1-{3-[7-(difluoromethyl)-6-(1-methyl-1H-pyrazol-4-yl)-3,4-dihydroquinolin-1(2H)-yl]-1-(oxan-4-yl)-1,4,6,7-tetrahydro-5H-pyrazolo[4,3-c]pyridin-5-yl}ethan-1-one 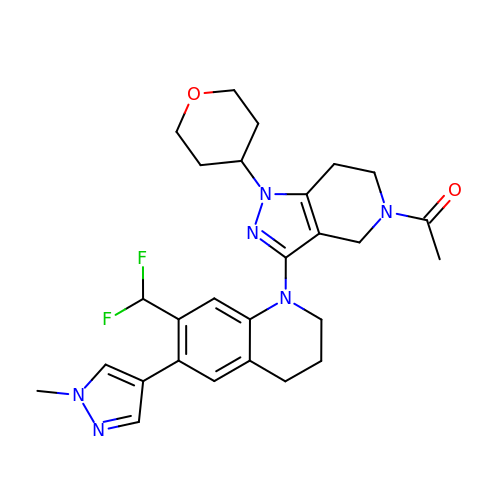| C27 H32 F2 N6 O2 | LWXLECMNBTVASW-UHFFFAOYSA-N>GPGSCPTHADSLNNLANIKREQGNIEEAVRLYRKALEVFPEFAAAHSNLASVLQQQGKLQEALMHYKEAIRISPTFADAYSNMGNTLKEMQDVQGALQCYTRAIQINPAFADAHSNLASIHKDSGNIPEAIASYRTALKLKPDFPDAYCNLAHCLQIVCDWTDYDERMKKLVSIVADQLEKNRLPSVHPHHSMLYPLSHGFRKAIAERHGNLCLDKINVLHKPPYEHPKDLKLSDGRLRVGYVSSDFGNHPTSHLMQSIPGMHNPDKFEVFCYALSPDDGTNFRVKVMAEANHFIDLSQIPCNGKAADRIHQDGIHILVNMNGYTKGARNELFALRPAPIQAMWLGYPGTSGALFMDYIITDQETSPAEVAEQYSEKLAYMPHTFFIGDHANMFPHLKKKAVIDFKSNGHIYDNRIVLNGIDLKAFLDSLPDVKIVKMKCPDGGDNADSSNTALNMPVIPMNTIAEAVIEMINRGQIQITINGFSISNGLATTQINNKAATGEEVPRTIIVTTRSQYGLPEDAIVYCNFNQLYKIDPSTLQMWANILKRVPNSVLWLLRFPAVGEPNIQQYAQNMGLPQNRIIFSPVAPKEEHVRRGQLADVCLDTPLCNGHTTGMDVLWAGTPMVTMPGETLASRVAASQLTCLGCLELIAKNRQEYEDIAVKLGTDLEYLKKVRGKVWKQRISSPLFNTKQYTMELERLYLQMWEH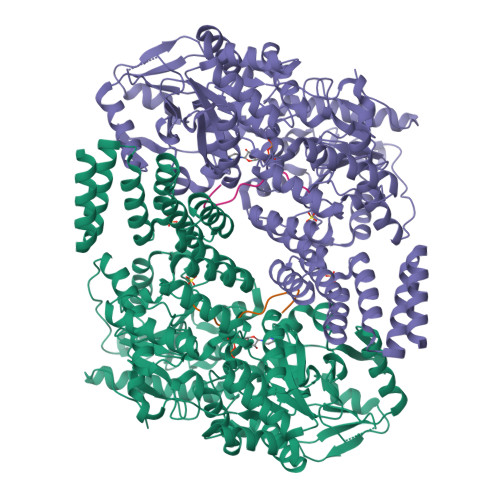YAAGNKPDHMIKPVE[2x];>[2x]YPGGSTPVSSANMM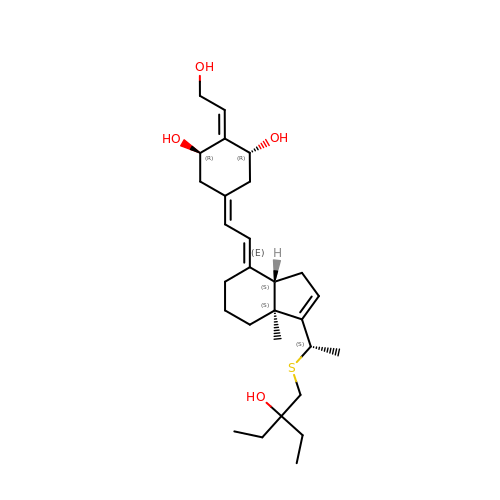(1R,2Z,3R,5E,7E)-17-{(1S)-1-[(2-ethyl-2-hydroxybutyl)sulfanyl]ethyl}-2-(2-hydroxyethylidene)-9,10-secoestra-5,7,16-triene-1,3-diol | C28 H44 O4 S | PIRFBNFXEQEXIT-XXUXJEHWSA-N> MASAAVANYEEE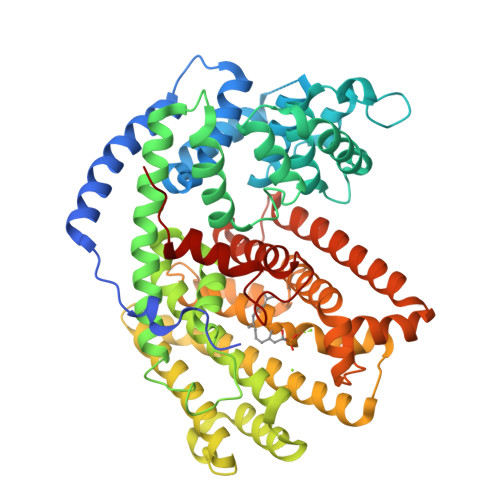IVRPVADFSPSLWGDQFLSFSIDNQVAEKYAKEIEALKEQTRNMLLATGMKLADTLNLIDTIERLGISYHFEKEIDDILDQIYNQNSNCNDLCTSALQFRLLRQHGFNISPEIFSKFQDENGKFKESLASDVLGLLNLYEASHVRTHADDILEDALAFSTIHLESAAPHLKSPLREQVTHALEQCLHKGVPRVETRFFISSIYDKEQSKNNVLLRFAKLDFNLLQMLHKQELAQVSRWWKDLDFVTTLPYARDRVVECYFSALGVYFEPQYSQARVMLVKTISMISIVDDTFDAYGTVKELEAYTDAIQRWDINEIDRLPDYMKISYKAILDLYKDYEKELSSAGRSHIVCHAIERMKEVVRNYNVESTWFIEGYTPPVSEYLSNALATTTYYYLATTSYLGMKSATEQDFEWLSKNPKILEASVIICRVIDDTATYEVEKSRGQIATGIECCMRDYGISTKEAMAKFQNMAETAWKDINEGLLRPTPVSTEFLTPILNLARIVEVTYIHNLDGYTHPEEVLKPHIINLLVDSIKI>[4x]MSNCQYKIYPPLGIARVGNGPAIKPLSLSTPEVPWAHLYDTNVQYLVTQQELEQLLEEAFGGNVINEISQIKTKLDERKAEKFKQEEIETITGLLGLSHLVPQQQLSRSLDNLELKSTKDSDDIVQQIKGALLKVLSDHYLHAVKKQAQNFYIYKCDEQGNPVEKLKLTDGDKVTWRVEVANKKSFWYDYNNALDLSLHTQGSGNLSKNVSKHRLAPAMTAKRRNPNVITNSLRKQLVISSQGSVSSDNNTQVPLRGKFPANEPDTNNRLSDLLNLQERHNVLQGSIECDNEGVLRFYAGNGISQALSPSSLNTDAADNSNWFDDICDGRVTAVVELKNGDTFEIQDEQSSAWVA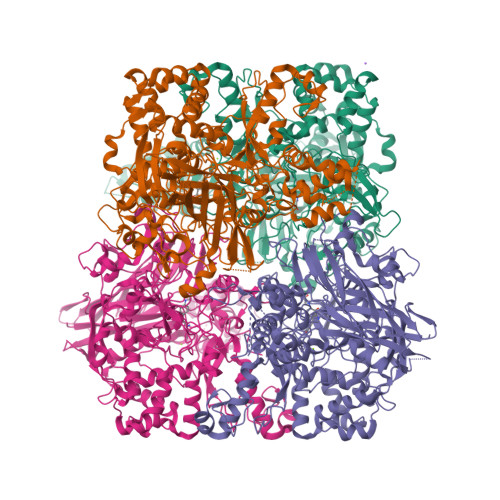TTPPDYAPQIEPIVTMYDMVSGAALKEQDLDNLTTQFSDVFPILYRLYRMQWVNQADFTDNAVNTQIRELNSELGFAQLLDNSASAKSLREGIFNQFRNPLFDQDIDVDDPGQSSNEWVSNSRIIPSKDETNIAAKPATSSLKLPFYPNDGIDYPGSPVQWFAIPPFMYQHLQNWAAGDFSVTQVEKESANTIEELGLFYSEQFKNSPNSALLCARGALDALYGGGFHPGVELTWPMRHNLIYSQNDYVSSVTPEINLLGLREFRLKQDLQGLNSPNMYQDFGHVIAVDNVTASIDPNSDAAWLWRSTPGDLTKWMGIPWQSDAASCQAVYTPEDFPIPSWXAANLPVHVLPLARYNKFKDSQSADLPEINGMTHSIAQGMSEETFEHLRLEQFSQRLDWLHTADLGFVGYHAEGGYTNGLIQMVSQWKNMAMVMARPVENPGSSGIPNVVYVAYSQADKD> MAPKATLVKKFKGLAVGVGALLAAPPIMGLASYAVNGISSYLSITINSTTYDFAPLAQAVMVFGGIGLVAYGLHRILGRGL

An excellent model for such studies is the non-enveloped bacilliform virus APBV1 infecting the archaeon Aeropyrum pernix that has the highest optimal growth temperature, 90 °C, among aerobic hyperthermophiles. The double-stranded, circular DNA genome of the virus (5.3 kbp) is among the smallest known dsDNA genomes. It encodes for the major capsid protein (MCP) VP1 (8.3 kDa) in addition to three minor capsid proteins VP2 (9.7 kDa), VP3 (11.2 kDa), and VP4 (21.4 kDa). To study the molecular basis of the extreme temperature resistance of APBV1, we have determined the three-dimensional structure of the purified APBV1 virion using electron cryomicroscopy (cryo-EM) to ~3-Å resolution.

Two-dimensional image classification of the segments and Fourier–Bessel analysis of power spectra calculated from 2D class averages revealed a defined helical symmetry (rise 6.10 Å, turn 16.55 degrees, 21.75 units per turn, pitch 133.7 Å), cyclic symmetry (C5), and the polar nature of the capsid structure. In the cryo-EM map, the fold of the VP1 glycoprotein and the density for most of the large amino acid side-chains were resolved, allowing us to build a VP1 atomic model de novo and refine it. VP1 is almost entirely α-helical, consisting of two long α-helices (α1, residues 5–42; α2, residues 53–77) linked by a type 1 beta hairpin (residues 43–52), and flexible termini (N-term, residues 1–4; C-term, 78–81). Two adjacent prolines (Pro25 and Pro26) mediate a kink in α1, which facilitated initial assignment of the sequence to the density. α2 is also curved at Gly66, but to lesser extent than α1. The arrangement of the VP1 subunits in the capsid resembles the blades of an impeller, with the small size of the VP1 protein, and more specifically the curvature of the VP1 α-helices α1 and α2, allowing very compact packing of subunits. Each VP1 subunit makes extensive hydrophobic contacts to six other neighboring VP1 subunits, resulting in a large interface area of 2916 Å2 (55.5% of the total solvent accessible area of the subunit). A large number of aliphatic residues pack closely with each other, with Leu14, Leu21, Ala24, Met28, Ala31, and Val35 of α1 packing against Met61, Leu68, Val69, Leu73, and Ile76 of α2 to form a very tight hydrophobic interface. Our analysis suggests that this interface contributes to APBV1 stability at high temperature. VP1 is glycosylated, and sequence analysis using NetNGlyc13 revealed an N-linked glycosylation sequon (46-NST-50) located at the tip of the loop region. Although the density map does not direct assignment of the VP1–DNA contacts, or an unambiguous determination of the DNA conformation, it suggests that the DNA follows the positively charged helical tracks formed by the VP1 residues Lys9 and Arg79 exposed on the inner surface of the helical capsid.>MAFKRAIIFTSFNGFEKVSRTEKRRLAKIINARVSIIDEYLRAKDTNASLDGQYRAFLFNDESPAMTEFLAKLKAFAESCTGISIDAWEIEESEYVRLPVERRDFLAAANGKEIFKI[2x];>GEIEKRQEENRKDREKAAAKFREYFPNFVGEPKSKDILKLRLYEQQHGKCLYSGKEINLGRLNEKGYVEIDHALPFSRTWDDSFNNKVLVLGSENQNK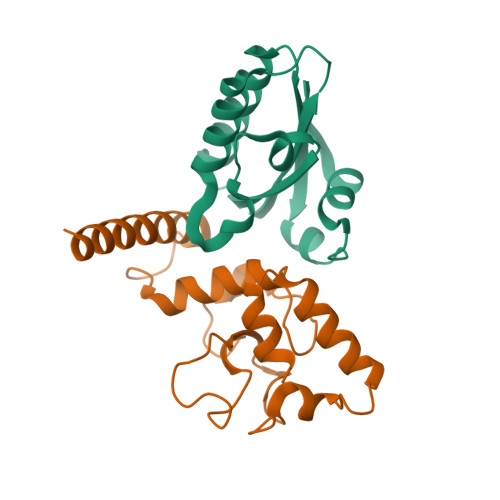GNQTPYEYFNGKDNSREWQEFKARVETSRFPRSKKQRILLQ[2x]> GSHMSVENIVNINE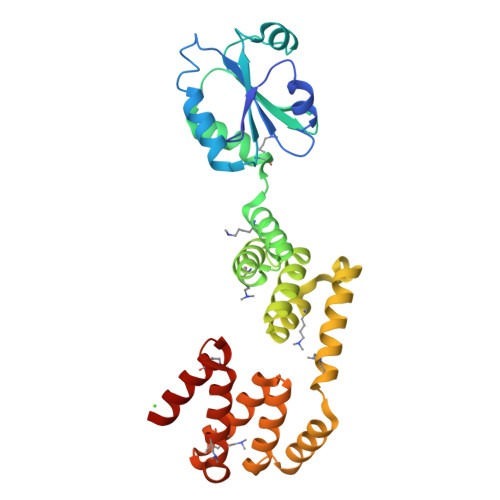SNLQQVLEQSMTTPVLFYFWSERSQHCLQLTPILESLAAQYNGQFILAKLDCDAEQMIAAQFGLRAIPTVYLFQNGQPVDGFQGPQPEEAIRALLDKVLPREEELKAQQAMQLMQESNYTDALPLLKDAWQLSNQNGEIGLLLAETLIALNRSEDAEAVLKTIPLQDQDTRYQGLVAQIELLKQAADTPEIQQLQQQVAENPEDAALATQLALQLHQVGRNEEALELLFGHLRKDLTAADGQTRKTFQEILAALGTGDALASKYRRQLYALLY The CCR4-NOT deadenylase complex plays a central role in bulk mRNA degradation by catalysing the removal of mRNA poly(A) tails, which is the first step in general mRNA decay. The CCR4-NOT complex consists of several structurally and functionally distinct modules, which assemble around the NOT1 scaffold subunit1. The CAF40 and NOT modules have no catalytic activity and have been implicated in mediating interactions with RNA-associated proteins that recruit the CCR4-NOT complex to their targets. Among these sites, we identify a short linear motif (SLiM) that is necessary and sufficient to mediate direct binding to the CAF40 subunit of the CCR4-NOT complex.

To elucidate the molecular principles underlying the recruitment of CAF40 by Dm Roquin, we sought to determine the crystal structure of the CBM peptide bound to the Dm and Hs CAF40 ARM domains, which exhibit 81% identity. However, only the complex containing Hs CAF40 yielded well-diffracting crystals, from which we obtained a structure at 2.15 Å resolution. The CBM peptide folds into an amphipathic helix (residues 795–810) that runs centrally across the concave surface of CAF40 and binds to a conserved hydrophobic patch close to the previously postulated nucleic acid-binding groove. The amphipathic helix of the CBM peptide lies almost parallel to helices α5, α8 and α11 and it uses residues M798, L801, L805, I808 and V809 on its hydrophobic side to interact with CAF40 residues Y134, L137, G141, G144 and A145 (helix α8) and L177, T180, V181 and F184 (helix α11). Furthermore, I793 anchors the N-terminal extension of the CBM helix between CAF40 residues A84, R130, P131 and Y134, resulting in a total buried surface of 1903 Å2 that does not include any water molecules. Finally, the CBM peptide is fixed by two hydrogen bonds between N804 and the CAF40 residue Q98 (helix α5) and by a hydrogen bond from CAF40 N88 (helix α5) to the carbonyl oxygen of G791. The CAF40 residues R130 and K148 may have additional roles in anchoring the CBM peptide, but they have distinct orientations in the two copies of the complex. Importantly, binding of the CBM does not interfere with NOT1 binding, suggesting that Dm Roquin can interact with CAF40 in the context of the CCR4-NOT complex.

>GPHMLEREKIYQWINELSSPETRENALLELSKKRESVPDLAPMLWHSFGTIAALLQEIVNIYPSINPPTLTAHQSNRVCNALALLQCVASHPETRSAFLAAHIPLFLYPFLHTVSKTRPFEYLRLTSLGVIGALVKTDEQEVINFLLTTEIIPLCLRIMESGSELSKTVATFILQKILLDDTGLAYICQTYERFSHVAMILGKMVLQLSKEPSARLLKHVVRCYLRLSDNPRAREALRQCLPDQLKDTTFAQVLKDDTTTKRWLAQLVKNLQE[2x];>[2x]EGGIDSGMMLQLEKNLVDIVD>[8x]MRHPVVMGNWKLNGSKEMVVDLLNGLNAELEGVTGVDVAVAPPALFVDLAERTLTEAGSAIILGAQNTDLNNSGAFTGDMSPAMLKEFGATHIIIGHSERREYHAESDEFVAKKFAFLKENGLTPVLCIGESDAQNEAGETMAVCARQL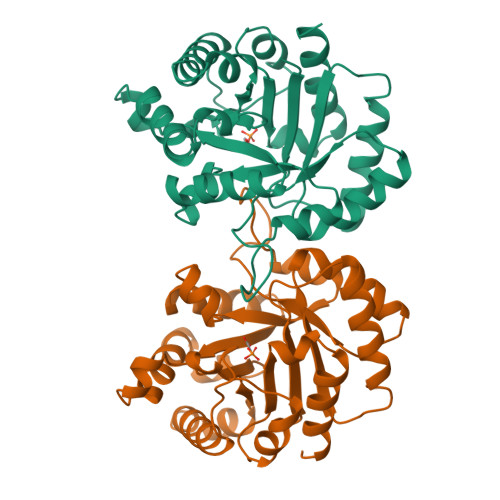DAVINTQGVEALEGAIIAYEPIWAIGTGKAATAEDAQRIHAQIRAHIAEKSEAVAKNVVIQYGGSVKPENAAAYFAQPDIDGALVGGAALDAKSFAAIAKAAAEAKA> AALGPSSQNVTEYVVRVPKNTTKKYNIMAFNAADKVNFATWNQARLERDLSNKKIYQEEEMPESGAGSEFNRKLREEARRKKYGIVLKEFRPEDQPWLLRVNGKSGRKFKGIKKGGVTENTSYYIFTQCP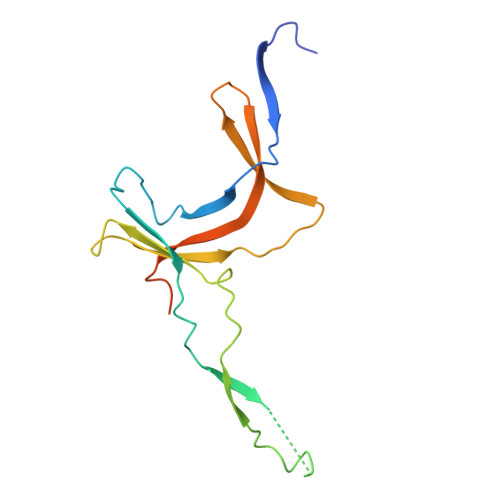DGAFEAFPVHNWYNFTPLARHRTLTAEEAEEEWERRNKVLN>MAWSHPQFEKGHMNDANIADVVTKVLGEYGAPGAVSVAALTAKSPDGKSNSSADADVVARMVAKAIRDHAGTAQPSGNAATSSAAVSDGVFETMDAAVEAAALAQQQYLLCSMSDRARFVQGIRDVILNQDTLEKMSRMAVEETGMGNYEHKLIKNRLAGEKTPGIEDLTTDAFSGDNGLTLVEYSPFGVIGAITPTTNPTETIVCN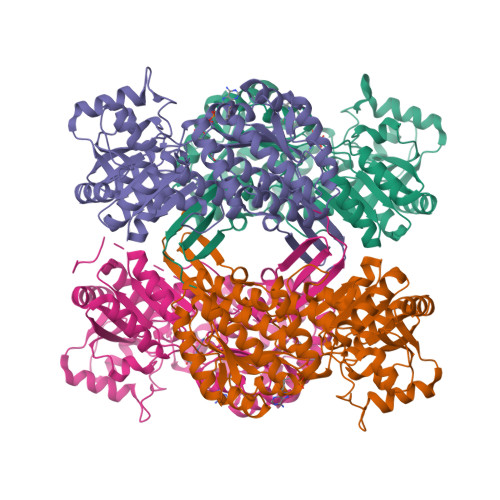SIGMLAAGNSVVFSPHPRARQVSLLLVRLINQKLAALGAPENLVVTVEKPSIENTNAMMAHPKVRMLVATGGPAIVKAVLSTGKKAIGAGAGNPPVVVDETANIEKAACDIVNGCSFDNNLPCVAEKEIIAVAQIADYLIFNLKKNGAYEIKDPAVLQQLQDLVLTAKGGPQTKCVGKSAVWLLSQIGISVDASIKIILMEVPREHPFVQEELMMPILPLVRVETVDDAIDLAIEVEHDNRHTAIMHSTDVRKLTKMAKLIQTTIFVKNGPSYAGLGAGGEGYSTFTIAGPTGEGLTSAKSFARRRKCVMVEALNIR[8x]> MTPNLQLYNKAYETLQGYGFPVISRKEMQQEIPYPFFVIKMPESNRSKYTFDSYSGDTNLVIDIWSVSDDLGHHDGLVKRCIDDLTPSVKTND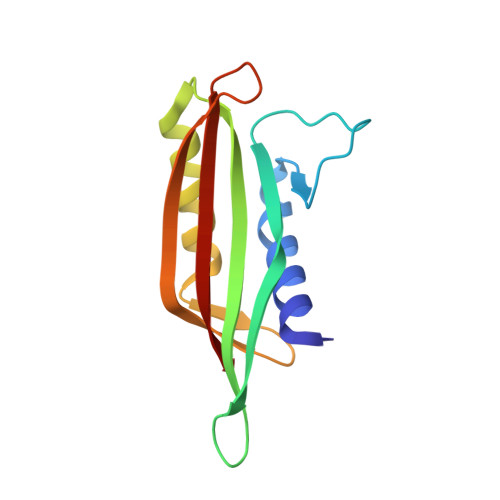YDFEEDDTNITQLVDDTTNQELLHTSITISYKTF> MKVGQDKVVTIRYTLQVEGEVLDQGELSYLHGHRNLIPGLEEALEGREEGEAFQAHVPAEKAYGPHDPEGVQVVPLSAFPEDAEVVPGAQFYAQDMEGNPMPLTVVAVEGEEVTVDFNHPLAGKDLDFQVEVVKVREATPEELLHGHAHPSGHHHHHH;> KMKPFIFGARNKVHIYX

Peptidyl-prolyl isomerases (PPIases) catalyze cis/trans isomerization of peptidyl-prolyl bonds, which is often rate-limiting for protein folding. SlyD is a two-domain enzyme containing both a PPIase FK506-binding protein (FKBP) domain and an insert-in-flap (IF) chaperone domain. In order to improve our understanding of the mechanism of SlyD and of FKBPs in general, we set out to analyze the kinetics, energetics, and structural basis for substrate binding and inhibition of SlyD from Thermus thermophilus (TtSlyD) using 15-residue-long unmodified peptides, which we reasoned would be better mimics of natural unfolded protein substrates than the traditionally used 4-nitroanilide tetrapeptides. In total, we obtained five structures of TtSlyDFL and three of TtSlyDΔIF at a maximum resolution of up to 1.4 Å.

To study the length dependency, we used variants of the S2 peptide extended or truncated with up to eight residues. Extension of the peptide had minor to moderate effects on the affinity for the IF domain (up to threefold higher) and the FKBP domain (up to threefold lower). A peptide is bound to the IF domain in four structures: TtSlyDFL:S2, TtSlyDFL:S2-W23A, TtSlyDFL:S2-plus, and TtSlyDFL:T1. The binding site consists of a highly hydrophobic groove comprising V74, F79, F91, L103, V115, and F117, as well as the edge of the β8–β9 hairpin. Interestingly, although the binding mode is variable, three aspects are shared for all structures: (i) the peptides bind to the β8–β9 hairpin through β-strand augmentation with two to four hydrogen bonds, (ii) the peptides generally insert two hydrophobic side chains into the binding groove as detailed above, and (iii) peptide binding does not perturb the hydrophobic groove.> SNA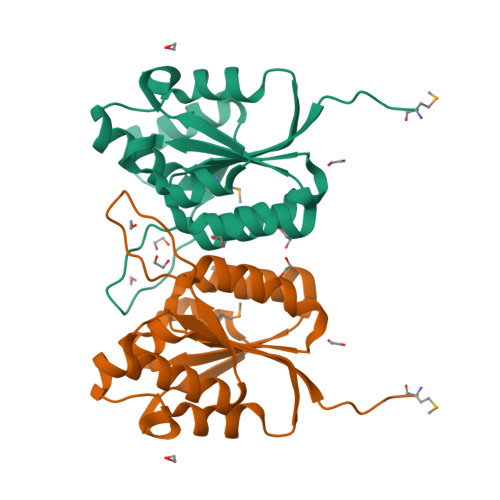MQSDHKEKIAILVDVQNVYYTCREAYRSNFDYNQFWYVATQEKEVVSAKAYAIASNDPKQRQFHHILRGVGFEVMLKPYIQRRDGSAKGDWDVGITLDAIEIAPDVDRVILVSGDGDFSLLVERIQQRYNKKVTVYGVPRLTSQTLIDCADNFVAIDDDFLL> LDNSYKMNHKRRGLCLIINNKNFDRKTGMKTRNGTDKDAENLEKTFKSLGFEVKVYNDLTAEEMQETLQ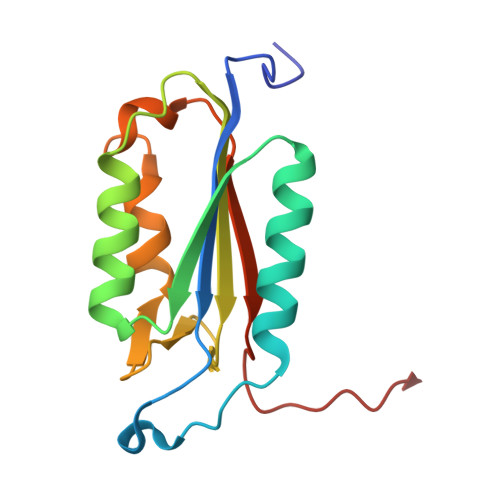EVSKEDHSDSDCFVCVLLSHGEEGLVYGTDGKIEIQELTSLFKGDKCQSLVGKPKLFFIQACRGDELDSGVEV> GPGAPNVLNWEQVQRLDGILSETIPIHGRGNFPTLELQPSLIVKVVRRRLAEKRIGVRDVRLNGSAASHVLHQDSGLGYKDLDLIFCADLRGEGEFQTVKDVVLDCLLDFLPEGVNKEKITPLTLKEAYVQKMVKVCNDSDRWSLISLSNNSGKNVELKFVDSLRRQFEFSVDSFQIKLDSLLLFYECSENPMTETFHPTIIGESVYGDFQEAFDHLCNKIIATRNPEEIRGGGLLKYCNLLVRGFRPASDEIKTLQRYMCSRFFIDFSDIGEQQRKLESYLQNHFVGLEDRKYEYLMTLHGVVNESTVCLMGHERRQTLNLITMLAIRVLADQNV;> GPGAPDEVIDEEVNIEFEAYSLSDNDYDGIKKLLQQLFLKAPVNTAELTDLLIQQNHIGSVIKQTDVSEDSNDDMDEDEVFGFISLLNLTERKGTQCVEQIQELVLRFCEKNCEKSMVEQLDKFLNDTTKPVGLLLSERFINVPPQIALPMYQQLQKELAGAHRTNKPCGKCYFYLLISKTFVEAGKNNSKKKPSNKKKAALMFANAEEEFFYEEQGKPEVLGGPDTRRGLEPVPIQHNGGSRGQVTALVSLKAGLIQSRSTLSDFQGTFMTVGIALS

The FAM46 (also known as TENT5) proteins are noncanonical poly(A) polymerases (PAPs) implicated in regulating RNA stability. Here, we report that the nuclear protein BCCIPα, but not the alternatively spliced isoform BCCIPβ, binds FAM46 and inhibits their PAP activity. Unexpectedly, our structures of the FAM46A/BCCIPα and FAM46C/BCCIPα complexes show that, despite sharing most of the sequence and differing only at the C-terminal portion, BCCIPα adopts a unique structure completely different from BCCIPβ. A helix-loop-helix segment in BCCIPα inserts into the active site cleft of FAM46, thereby inhibiting the PAP activity.

To understand how BCCIPα binds the FAM46 proteins and inhibits their PAP activity, we sought to solve the crystal structure of a FAM46/BCCIPα complex. After extensive screening of various constructs of BCCIPα and the FAM46 family members, we were able to obtain crystals of the complex between FAM46A and BCCIPα-ΔS, which contains deletions in flexible loop regions. Strikingly, the structure showed that BCCIPα adopts a structural fold that is completely different from the structure of BCCIPβ published previously (see details below). The structure of the FAM46A/BCCIPα complex for the first time revealed the fold of BCCIPα. Furthermore, A DALI search of the protein structural database suggested that the fold of BCCIPα is unique, as the search failed to find any protein with substantial similarity to BCCIPα. In contrast, while the β sheet in BCCIPα also starts with strand β1 at one edge, the strands are arranged in space in the order of 1-6-5-3-7-4-2. However, in our structure, this region forms two β strands, strands 6 (residues 296 to 303) and 7 (residues 316 to 320). Consistent with the published structures of FAM46B and FAM46C, FAM46A in the FAM46A/BCCIPα complex adopts the same bi-lobal structure, with the PAP enzymatic active site residues in the cleft between the two lobes. The N-terminal lobe contains a large β sheet that is covered by several α helices on one side, whereas the other side of the β sheet faces the catalytic site cleft, presenting the conserved catalytic residues, including Gly122, Ser123, Asp139, Asp141 (for binding ATP and Mg2+), and Glu215 (the catalytic base), to form the active site of the enzyme. Our observation that BCCIPα can promote the nuclear localization of FAM46 is consistent with the structure of the complex where the NLS is available for driving their nuclear translocation as it is not occupied by the binding interface with FAM46.> VEWTDSERAIITSIFSNLDYEEIGRKS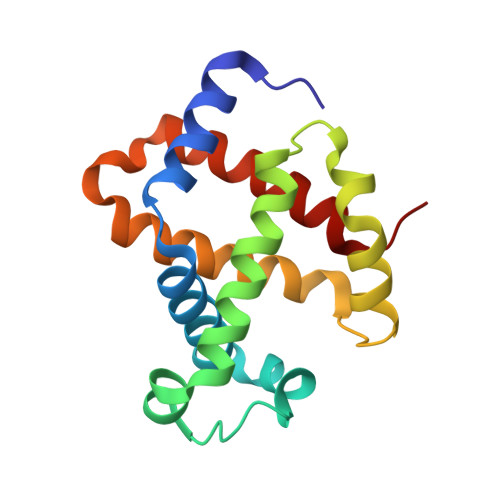LCRCLIVYPWTQRYFGAFGNLYNAETILANPLIAAHGTKILHGLDRALKNMDDIKNTYAELSLLHSDKLHVDPDNFRLLADCLTVVIAAKMGSAFTVDTQVAWQKFLSVVVSALGRQY> GSHMEKTGLHVHEKIKHMVKNYGTMITGIPAEILGQNEAEISVGYVKKMGNMKENIAEVVRKSEMTQPTNSAGKASNEVCDLLLGTEGASEFEKSSYQVLSGDGSNLKGSLPNKNLLVRVEMDRFNAPQKYQKIKREEFNPETAEKNKIYLLEDQLVYLDIFGKVIDLGQTSDTCHRLFNAITTPFYQNYILYDEYIDPEESAEEAAMFEM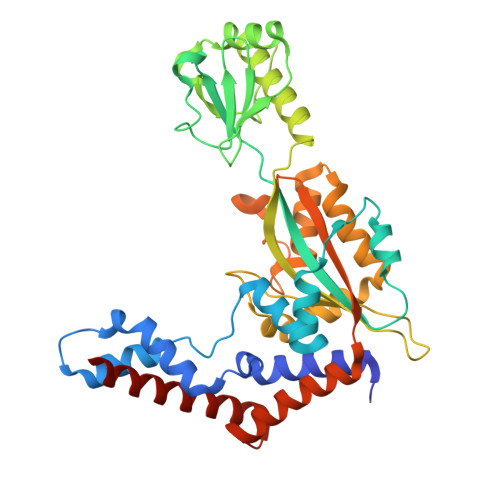GEIVKAKMKNIDCWTATHSFTIFVPESDSEDTRTLYPYQAYWTSHTLQQWFSGDKDEKLSRLGIDGYIEKLALLGTTTDSKIRSSIYGELFSPPGKEHVFCTGMNEKFSPLRVKFKVTEVNPEIALQNLEEVQEFIDTNYPGENAKDQCELYKIKAQEAMTKQLEMRLLIE>SNAMPMNISNTKERILA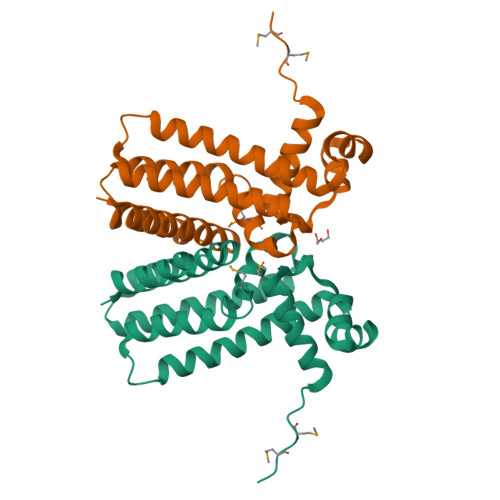VAEALIQKDGYNAFSFKDIATAINIKTASIHYHFPSKEDLGVAVISWHTDKIAAVLSDISNNSSLSAKEKIQKFFDAILTLTYNSENKMCLGGMFASDFQSLPVSIQNQAKKFFELIIEWLKGVLETNGYDNESSLSLAKQIISLVEGGLLLARLYGDETFLEGVRHFIDQTIK[8x]> GAMGMIDIHSHIVFDVDDGPKSREESKALLAESYRQGVRTIVSTSHRRKGMFETPEEKIAENFLQVREIAKEVASDLVIAYGAEIY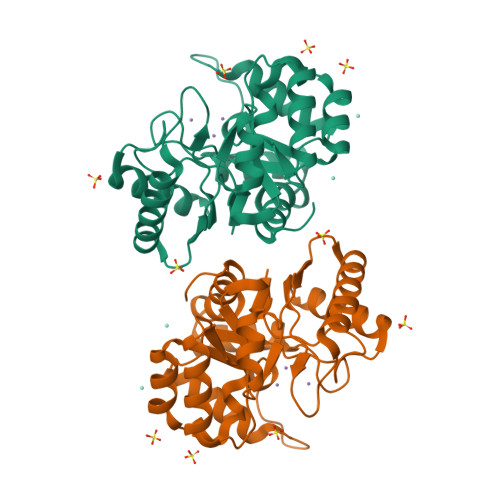YTPDVLDKLEKKRIPTLNDSRYALIEFSMNTPYRDIHSALSKILMLGITPVIAHIERYDALENNEKRVRELIDMGCYTQVNSSHVLKPKLFGERYKFMKKRAQYFLEQDLVHVIASDMHNLDGRPPHMAEAYDLVTQKYGEAKAQELFIDNPRKIVMDQLI>[2x]GPSTVQELDLAGITDSGLRADYIASSQLFRKIGRGR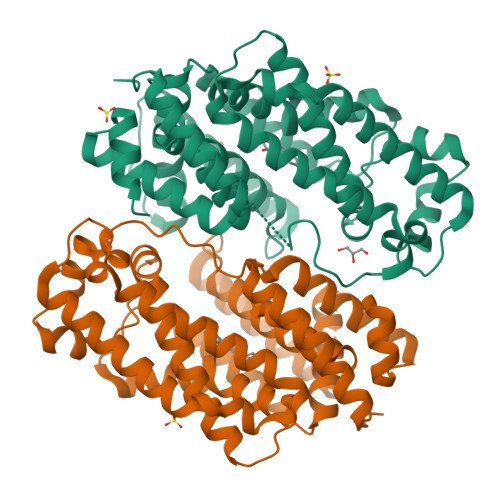FLGRYMMHPAKRPYFDTFFSFVCYIDDLADDINLSVDVRARRLDEWQRTYLAIAKGEDEHPLSLSEQTDAALARALVHTLRTWDLPYLRVPEFVDGHRKALTTYEYADQEELDDFLETVTLLPAIWINQIFEPISEDAEELCRHTITAFQLLDFIWDLREDLDLGRLYLPLDHLARFGLTRADLDRQIGSGYISDALRELIQFEIDIAREHMNAGRSWPQTLHPTARIFMETDIQTHDSMFPEMIKDDYAFFKSPLDFVSGRMIPRTAKAIARARKANQQATRAGYRIRPPYRGTEA> NLQSQFFIEHILQILPHRYPMLLVDRITELQANQKIVAYKNITFNEDVFNGHFPNKPIFPGVLIVEGMAQSGGFLAFTSLWGFDPEIAKTKIVAFMTIDKVKFRIPVTPGDRLEYHLEVLKHKGMIWQ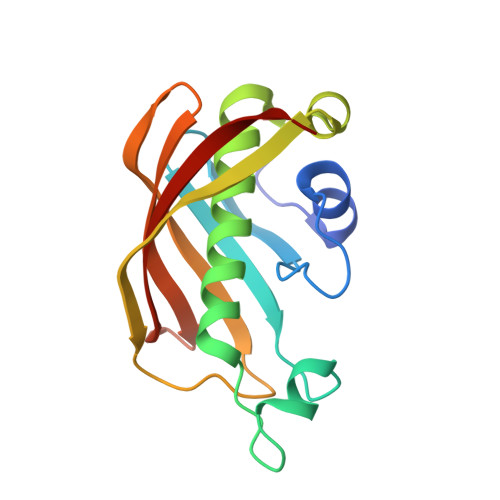VGGTAQVDGKVVAEAELKAMIAERE>MSYPATRAEQVVDTLHGVQVADPYRWLEDEKAPEVQTWMTAQNAHAREALAKFPGREALAARFKELFYTDSVSTPSRRNGRFFYVRTHKDKEKAILYWRQGESGQEKVLLDPNGWSKDGTVSLGTWAVSWDGKKVAFAQKPNAADEAVLHVIDVDSGEWSKVDVIEGGKYATPKWTPDSKGFYYEWLPTDPSIKVDERPGYTTIRYHTLGTEPSKDTVVHERTGDPTTFLQSDLSRDGKYLFVYILRGWSENDVYWKRPGEKDFRLLVKGVGAKYEVHAWKDRFYVLTDEGAPRQRVFEVDPAKPARASWKEIVPEDSSASLLSVSIVGGHLSLEYLKDATSEVRVATLKGKPVRTVQLPGVGAASNLMGLEDLDDAYYVFTSFTTPRQIYKTSVSTGKSELWAKVDVPMNPEQYQVEQVFYASKDGTKVPMFVVHRKDLKRDGNAPTLLYGYGGFNVNMEANFRSSILPWLDAGGVYAVANLRGGGEYGKAWHDAGRLDKKQNVFDDFHAAAEYLVQQKYTQPKRLAIYGGSNGGLLVGAAMTQRPELYGAVVCAVPLLDMVRYHLFGSGRTWIPEYGTAEKPEDFKTLHAYSPYHHVRPDVRYPALLMMAADHDDRVDPMHARKFVAAVQNSPGNPATALLRIEANAGHGGADQVAKAIESSV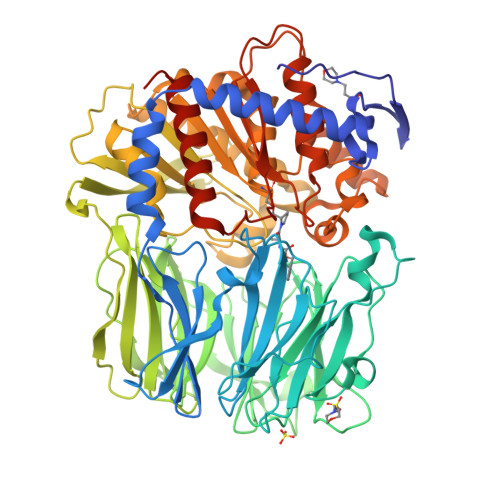DLYSFLFQVLDVQGAQGGVAAQGRHHHHHH[2x]>[6x]MTSAEMTSPNNNSEHQAIAKMRTMIEGFDDISHGGLPIGRSTLVSGTSGTGKTLFSIQFLYNGIIEFDEPGVFVTFEETPQDIIKNARSFGWDLAKLVDEGKLFILDASPDPEGQEVVGGFDLSALIERINYAIQKYRARRVSIDSVTSVFQQYDASSVVRRELFRLVARLKQIGATTVMTTERIEEYGPIARYGVEEFVSDNVVILRNVLEGERRRRTLEILKLRGTSHMKGEYPFTITDHGINIFPLGAMRLTQRSSNVRVSSGVVRLDEMCGGGFFKDSIILATGATGTGKTLLVSRFVENACANKERAILFAYEESRAQLLRNAYSWGMDFEEMERQNLLKIVCAYPESAGLEDHLQIIKSEINDFKPARIAIDSLSALARGVSNNAFRQFVIGVTGYAKQEEITGLFTNTSDQFMGAHSITDSHIDTITDTIILLQYVEIRGEMSRAINVFKMRGSWHDKAIREFMISDKGPDIKDSFRNFERIISGSPTRITVDEKSELSRIVRGVQEKGPES

The circadian clock of the cyanobacterium Synechococcus elongatus can be reconstituted in vitro by three proteins, KaiA, KaiB and KaiC. Homo-hexameric KaiC displays kinase, phosphatase and ATPase activities; KaiA enhances KaiC phosphorylation and KaiB antagonizes KaiA. The crystal structure of KaiC from S. elongatus revealed a hexamer in the shape of a double doughnut with approximate dimensions 100×100 Å, whereby the N-terminal CI and C-terminal CII halves of subunits are joined by a 15-amino acid linker. Two phosphorylation sites (P-sites), T432 and S431 that are both located in the CII half were identified in KaiC.

To analyze the phosphorylation patterns of KaiC P-site mutants and to visualize potential conformational variations in the vicinity of bound ATP and residues 432 and 431 at hexamer subunit interfaces, we determined crystal structures of the S. elongatus KaiC single mutants T432A (TSa), S431A (TaT), S431D (TdT), and T426N (nST) and the double mutants T426A/T432A (aSa) and S431A/T432E (Tae). b KaiC mutations xyz or mutants KaiCxyz are sequentially shown in order of sites x = 426, y = 431, and z = 432 where the wild-type residue is in upper case and mutated residues are shown in lower case, i.e. Tsa or KaiCTSa, where the residue at position 426 is T, the residue at position 431 is S, and the residue at position 432 is mutated to A. The structures of the TdT, nST and aSa mutants provide further support for the conclusion that T432 is the principal phosphorylation site because it lies closest to the γ-phosphate. The combined structural data expose subtle changes in the orientations of the H423-I433 loop region harboring phosphorylated residues relative to the γ-phosphate of ATP compared with the structure of wt-KaiC.>MRLTNLLSLTTLVALAVAVPDFYQKREAVSSKEAALLRRDASAECVSNENVEIEAPKTNIWTSLAKEEVQEVLDLLHSTYNITEVTKADFFSNYVLWIETLKPNKTEALTYLDEDGDLPPRNARTVVYFGEGEEGYFEELKVGPLPVSDETTIEPLSFYNTNGKSKLPFEVGHLDRIKSAAKSSFLNKNLNTTIMRDVLEGLIGVPYEDMGCHSAAPQLHDPATGATVDYGTCNINTENDAENLVPTGFFFKFDMTGRDVSQWKMLEYIYNNKVYTSAEELYEAMQKDDFVTLPKIDVDNLDWTVIQRNDSAPIRHLDDRKSPRLVEPEGRRWAYDGEEEYFSWMDWGFYTSWSRDTGISFYDITFKGERIVYELSLQELIAEYGSDDPFNQHTFYSDISYGVGNRFSLVPGYDCPATAGYFTTDTFEYDEFYNRTLSYCVFENQEDYSLLRHTGASYSAITQNPTLNVRFISTIGNYDYNFLYKFFLDGTLEVSVRAAGYIQAGYWNPETSAPYGLKIHDVLSGSFHDHVLNYKVDLDVGGTKNRASKYVMKDVDVEYPWAPGTVYNTKQIAREVLEKEDFNGINWPENGQGILLIESAEETNSFGNPRAYNIMPGGGGVHRIVKNSRSGPETQNW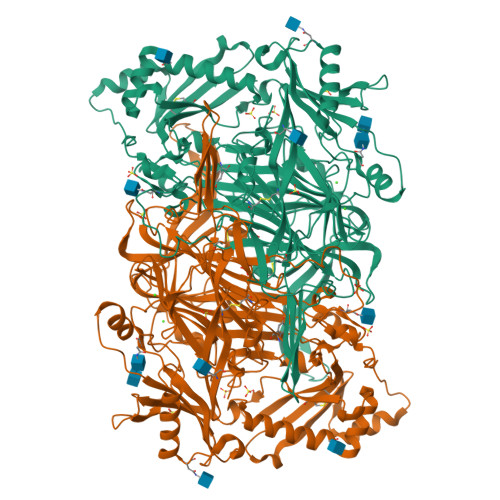ARSNLFLTKHKDEELRSSTALNTNALYDPPVNFNAFLDDESLDGEDIVAWVNLGLHHLPNSNDLPNTIFSTAHASFMLTPFNYFDSENSRDTTQQVFYTYDDETEESNWEFYGNDWSSCGLEVPEPNFEDYTYGRGTRINKKMTNSDEVY[4x]ADARs (adenosine deaminases that act on RNA) catalyze adenosine deamination within duplex RNA yielding inosine. ADARs are multidomain proteins with N-terminal double stranded RNA binding domains (dsRBDs) and C-terminal deaminase domains. Since the substrate for ADARs is an RNA duplex, the enzymes access the reactive adenosine using a base flipping mechanism. For instance, the nearest neighbor nucleotide preferences for ADARs show a strong bias against reaction at adenosines with a guanosine 5′ to the target adenosine (5′-GA sites).

Therefore, to gain greater insight into the structural basis for efficient editing by ADAR with a G:G pair adjacent to an editing site, we turned to X-ray crystallography to determine the atomic resolution structure of ADAR2-R2D E488Q bound to the GLI1 RNA substrate containing the G:G pair. We were able to grow protein–RNA crystals using the 32 bp azaN-containing duplex with the G:G pairing and ADAR2-R2D E488Q, which diffracted X-rays beyond 2.7 Å resolution. As we have seen with the related protein–RNA combination, the protein bound the RNA as an asymmetric homodimer with the deaminase domain of one monomer (monomer A) involved in direct RNA binding to the flipped-out azaN nucleoside. Importantly, the G:G pair adjacent to the editing site is well resolved with electron density that best fits a Gsyn:Ganti pair with the guanosine on the 5′ side of the azaN in a syn conformation with its Hoogsteen face accepting two hydrogen bonds from the Watson–Crick face of the guanosine on the opposing strand. The G:G pairing involves N1 to O6 and 2-amino to N7 hydrogen bonding seen in other Gsyn:Ganti pairs in RNA. The Gsyn:Ganti pair solves this apparent steric problem by inducing a change in the glycosidic bond angle at the 5′ G from anti to syn, moving the offending 2-amino group into the major groove where it does not clash with ADAR. However, the Gsyn:Ganti pair still presents a 2-amino group to the minor groove from the guide strand Ganti, which causes a slight shift in the base-flipping loop compared to the previous ADAR2-R2D – GLI1 structure. The α-carbon of Gly489 shifts ∼1.0 Å towards the edited strand. This shift can be accommodated because of the increased ribose-ribose spacing in a Gsyn:Ganti pair as seen in other structures. In the Gsyn:Ganti pair structure, only the pro-SP non-bridging oxygen interacts with Arg455, while in previous ADAR2–RNA complex structures, both non-bridging oxygens interact with the guanidino group of Arg455.

>[2x]GASLAQPPLPVLPPFPPPSGKNPVMILNELRPGLKYDFLSESGESHAKSFVMSVVVDGQFFEGSGRNKKLAKARAAQSALAAIFNLHLDQTPSRQPIPSEGLQLHLPQVLADAVSRLVLGKFGDLTDNFSSPHARRKVLAGVVMTTGTDVKDAKVISVSTGTKCINGEYMSDRGLALNDCHAEIISRRSLLRFLYTQLELYLNNKDDQKRSIFQKSERGGFRLKENVQFHLYISTSPCGDARIFSPHEPILEEPADRHPNRKARGQLRTKIESGQGTIPVRSNASIQTWDGVLQGERLLTMSCSDKIARWNVVGIQGSLLSIFVEPIYFSSIILGSLYHGDHLSRAMYQRISNIEDLPPLYTLNKPLLSGISNAEARQPGKAPNFSVNWTVGDSAIEVINATTGKDELGRASRLCKHALYCRWMRVHGKVPSHLLRSKITKPNVYHESKLAAKEYQAAKARLFTAFIKAGLGAWVEKPTEQDQFSLTP> CGYSDRVQQITLGNSTITTQEAANAVVCYAEWPEYLPDVDASDVNKTSKPDTSVCRFYTLDSKTWTTGSKGWCWKLPDALKDMGVFGQNMFFHSLGRSGYTVHVQCNATKFHSGCLLVVVIPEHQLASHEGGNVSVKYTFTHPGERGIDLSS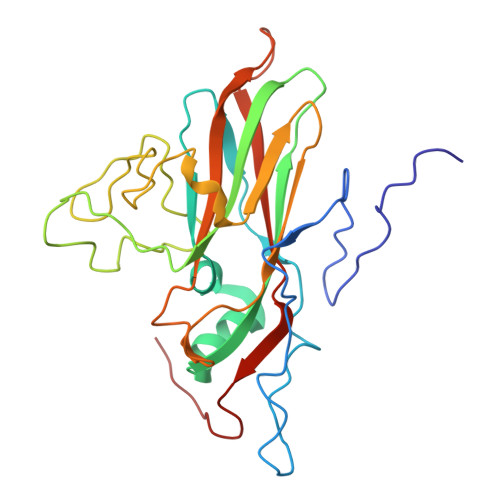ANEVGGPVKDVLYNMNGTLLGNLLIFPHQFINLRTNNTATIVIPYINSVPIDSMTRHNNVSLMVIPIAPLTVPTGATPSLPITVTIAPMCTEFSGIRSKSIVPQ>[2x]MIRKIYDKLVESHNEIKNQIYNIANYLKQEIQDKVNEYWNEYVINHEQSETCKFVAIDGGSFGRPMRIGIVYAVGAESVIGDNKGVKTLSEDGQIGIFKPGNDAQER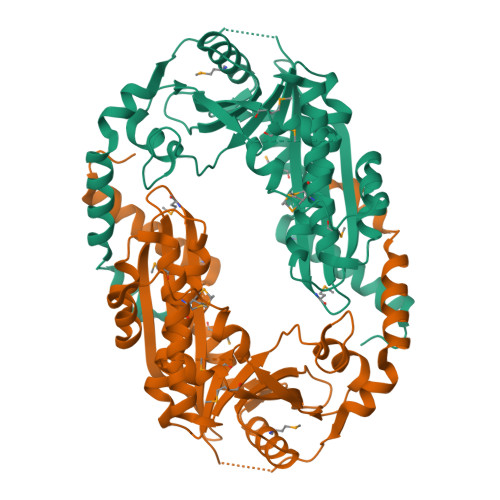ISLLMEALELSLALRDGSKGDYILMDGSLSKKIGNKVDIQQFSDEELKLIRNVDLNGIISIKDERKMRDLLMLLNQFLVSKIIEEYDGNVLWISKVSRGRDLFGTDYPDITVLELFTEKRGFSKLIIKNIDIEKISEIPEIEVLRKMEYTTFYTRLDNGKRVIRVDIVGRVDEKIVKEIMDRLSGVSIKGYPFPLLKAHMDVRFSAMDREKIIKLVGSKLHKDIEWWPSQFY> ACPAPPPGQPDIRAIGYYTDKAGSVIDPALQQQNKDATAPLDRYAADVARMSDDYLRNGDPAAAQCTLSWLGAWADDGAMLGQMIRVNNDQSFYMRQWMLDAVAMAYLKVHDQANPQQRARIDPWLQKLARANLAYWDNPKRRRNNHYYWGGLGVLATGLATDDDALWQAGHAAFQKGIDDIQDDGSLPLEMARGQRALHYHDYALAPLVMMAELARLRGQDWYASRNHAIDRLARRVIEGSRDPAWFNQHTGAAQLPLQASGWVEFYRLRSPDGGVFDAAHARGPFHSPRLGGDLTLMATHGIVRTPL

Unlike other PLs, Smlt1473 present in the clinically relevant Stenotrophomonas maltophilia strain K279a demonstrates a wide range of pH-dependent substrate specificities toward multiple, diverse polysaccharides: hyaluronic acid (pH 5.0), poly-β-D-glucuronic (celluronic) acid (pH 7.0), poly-β-D-mannuronic acid, and poly-α-L-guluronate (pH 9.0). To decode the pH-driven multiple substrate specificities and selectivity in this single enzyme, we present the X-ray structures of Smlt1473 determined at multiple pH values in apo and mannuronate-bound states as well as the tetra-hyaluronate-docked structure. We have built and refined the structures from residues A22-L330; electron density for other residues outside this range was either weak or absent. The structure is composed of 13 α-helical segments (α-1 to α-13) connected by 14 loops (L-1 to L-14) and two β-strands (β-1 and β-2) (Fig. 2, B and C (i and ii)).

To gain insight into this possibility, we analyzed the statistical distribution of B-factors in different apo structures at pH 5.0, 7.0, and 9.0, which were solved at comparable resolutions of 2.63, 2.20, and 2.45 Å, respectively. The protein is least flexible at acidic pH, most flexible at neutral pH, and has intermediate flexibility at basic pH. The pH 5.0 and 9.0 apo structures possess higher flexibility at the entry site than at pH 7.0. However, significant rotameric transitions of important substrate-binding residues such as K42, K162, R163, H221, and R312L have been observed at different pH values. At the exit site, K42 exhibits an altered orientation only in the pH 6.5 and 9.0 structures, whereas in pH 5.0 and pH 5.5 there is no change in orientation; interestingly, at pH 7.0 and 8.5 a lack of electron density precluded analysis of the residue orientation. For K162, the altered orientation was observed only for the pH 6.5 and 9.0 structures; for pH 7.0 and pH 8.5 a lack of electron density precluded analysis of residue orientation. For R163, pH 6.5, 7.0, and 9.0 structures have similar rotamers, in contrast to the pH 5.0 and 5.5 structures.> ICLEIKX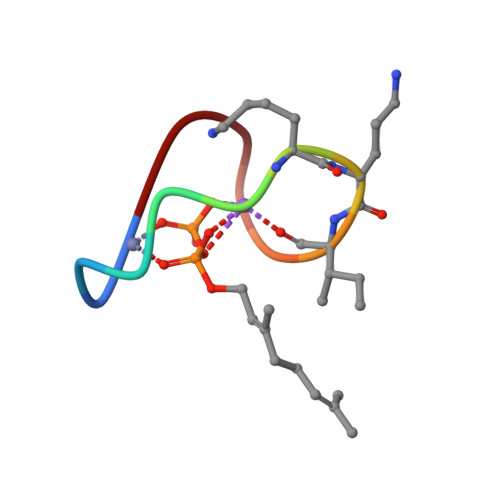IFHDN4-(4-{2-[(2,2-dimethylpropanoyl)amino]ethyl}piperidin-1-yl)thieno[3,2-d]pyrimidine-6-carboxamide 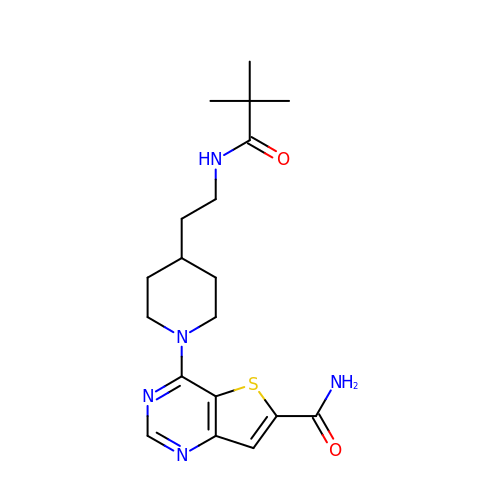| C19 H27 N5 O2 S | NSPKBHVNVJWICU-UHFFFAOYSA-N>GAMDMKTLTTISGHSKDNLALLKCLQGETKEKEFEISNVLPNHKMKEKLFRENKLKIDIDIEKDIFNYSRKNIQKIEFMPVNRLISQSEIDGIIGTLKEVLPTGQFTSGPFSKKLEEVIGDYLNKKYVIATSSGTDALMVSLLSIGIQPGDEVIMPANSFAATENAVLAIGAKPVFVDIDHKSYCIDPLKIEEAITQKTKCILPVHLYGKQCDMKRIREIADVYQLRIIEDACQAIGSSNLGEYGDIIILSFNPYKNFGVCGKAGAIVTNNENLAIRCNQY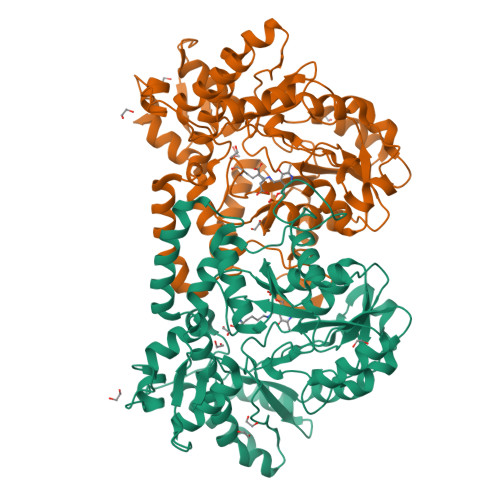SYHGFEVDKKNKKVLDFGFNSKIDNLQAAIGLERIKFLSYNNLKRVFLAQRYIRNLKELEDRELIKLPRMTEDNVWHLFPIRIINGRRDEVKNKLYQLYNIETDIYYPVLSHKHNTKLVKKNYMQDTLLNTEQVHKEILHLPLHPNMLLEEQNFVLEGLINVNK[8x]3-[3-(3-methylbut-2-enyl)-4-oxidanyl-phenyl]-5-[[3-(3-methylbut-2-enyl)-4-oxidanyl-phenyl]methylidene]-4-oxidanyl-furan-2-one | C27 H28 O5 | 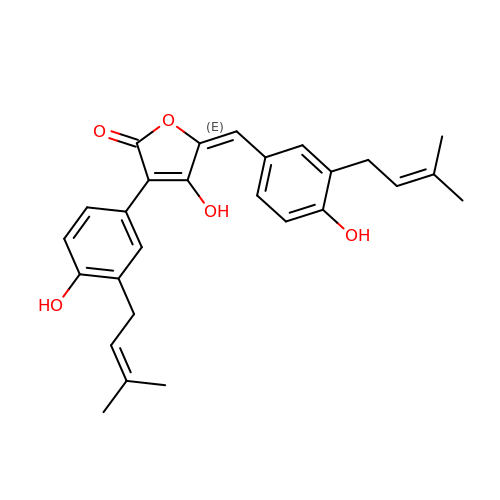LFDYHAWYVIBCDT-UHFFFAOYSA-N> MQIYEGKLTAEGLRFGIVASRFNHALVDRLVEGAIDCIVRHGGREEDITLVRVPGSWEIPVAAGELARKEDIDAVIAIGVLIRGATPHFDYIASEVSKGLANLSLELRKPITFGVITADTLEQAIERAGTKHGNKG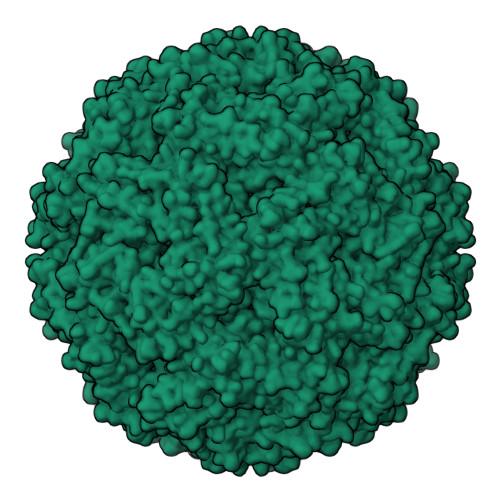WEAALSAIEMANLFKSLRWSHPQFEK>[2x]MSNISLIVGLGNPGSEYAQTRHNAGFWFVEQLADKYGITLKNDPKFHGISGRGNIEGHDVRLLLP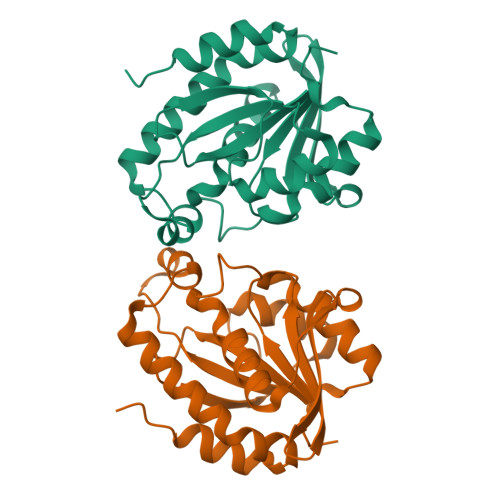MTYMNRSGQSVVPFSKFYQIAPEAILIAHDELDMNPGVIRLKTGGGHGGHNGLRDIVPHIGPNFHRLRIGIGHPGSKERVSGHVLGKAPSNEQSLMDGAIDHALSKVKLLVQGQVPQAMNQINAYKPA>LSSSPSEILQELGKGSTHPQPGVSPPAAPAAPGPKDGPGETDAFGNSEGKELVASGENKIKQGLLPSLEDLLFYTIAEGQEKIPVHKFITALKSTGLRTSDPRLKECMDMLRLTLQTTSDGVMLDKDLFKKCVQSNIVLLTQAFRRKFVIPDFMSFTSHIDELYESAKKQSGGKVADYIPQLAKFSPDLWGVSVCTADGQRHSTGDTKVPFCLQSCVKPLKYAIAVNDLGTEYVHRYVGKEPSGLRFNKLFLNEDDKPHNPMVNAGAIVVTSLIKQGVNNAEKFDYVMQFLNKMAGNEYVGFSNATFQSERESGDRNFAIGYYLKEK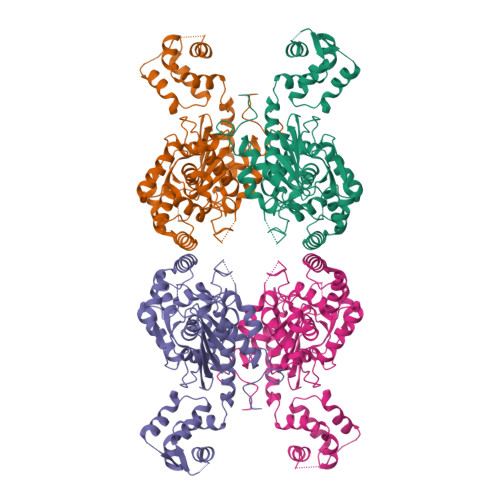KCFPEGTDMVGILDFYFQLCSIEVTCESASVMAATLANGGFCPITGERVLSPEAVRNTLSLMHSCGMYDFSGQFAFHVGLPAKSGVAGGILLVVPNVMGMMCWSPPLDKMGNSVKGIHFCHDLVSLCNFHNYDNLRHFAKKLDPRREGGDQRHSFGPLDYESLQQELALKETVWKKVSPESNEDISTTVVYRMESLGEKS[2x]>AEVPLPQLRAYTVDASWLQPMAPLQIADHTWQIGTEDLTALLVQTPDGAVLLDGGMPQMASHLLDNMKARGVTPRDLRLILLSHAHANHAGPVAELKRRTGAKVAANAESAVLLARGGSDDLHFGDGITYPPANADRIVMDGEVITVGGIVFTAHFMAGHTPGSTAWTWTDTRNGKPVRIAYADSLSAPGYQL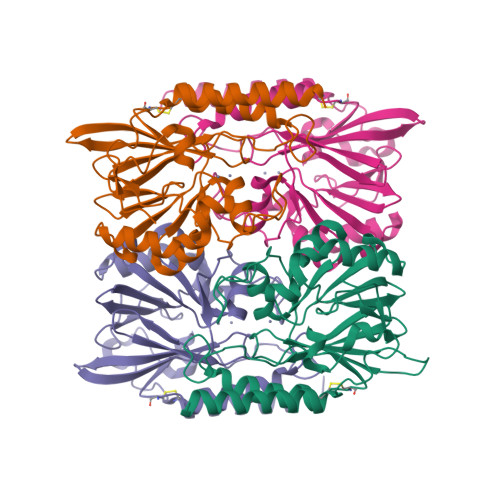QGNPRYPHLIEDYRRSFATVRALPCDVLLTPHPGASNWDYAAGARAGAKALTCKAYADAAEQKFDGQLAKETAGAR[4x]> SMEAEKQSDIKGTIAFDTHGNVIESTGVGSQRIEDIGDLSKVTLDAEGFAQVQGDSLLV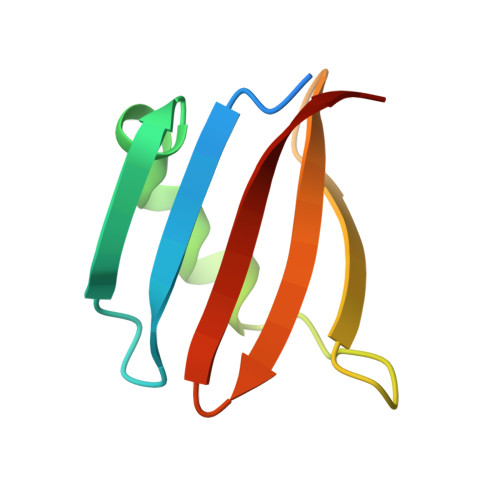HLYKRNDITLAVYTSAQ> GAMGSWNPKYDTRTLWTTPDTSPNCTIAQDKDSKLTLVLTKCGSQILANVSLIVVAGKYHIINNKTNPKIKSFTIKLLFNKNGVLLDNSNLGKAYWNFRSGNSNVSTAYEKAIGFMPNLVAYPKPSNSKKYARDIVYGTIYLGGKPDQPAVIKTTFNQETGCEYSITFNFSWSKTYENVEFETTSFTFSYIAQE;> MADFARSLSITTPEEMIEKAKGETAYLPCKFTLSPEDQGPLDIEWLISPADNQKVDQVIILYSGDKIYDDYYPDLKGRVHFTSNDLKSGDASINVTNLQLSDIGTYQCKVKKAPGVANKK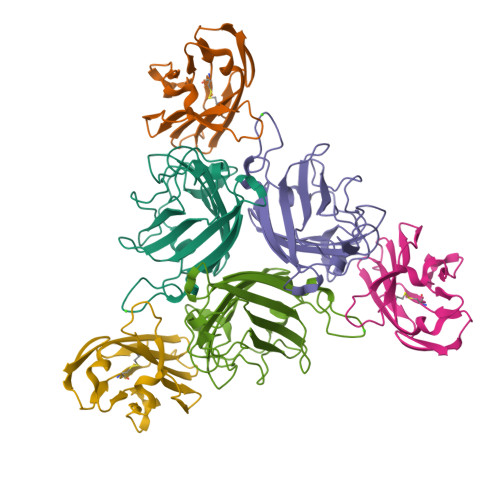IHLVVLVK>[2x]MKKNGKSQNQPLDFTQYAKNMRKDLSNQDICLEDGALNHSYFLTKKGQYWTPLNQKALQRGIELFGVGNWKEINYDEFSGKANIVELELRTCMILGINDITEYYGKKISEEEQEEIKKSNIAKGKKENKLKDNIYQKLQQMQ;>[2x]DDYLDRLPKSKKGLQGLLQDIEKRILHYKQLFFKEQNEIANGKRSMVPDNSIPICSDVTKLNFQALIDAQMRHAGKMFDVIMMDPPWQLSSSQP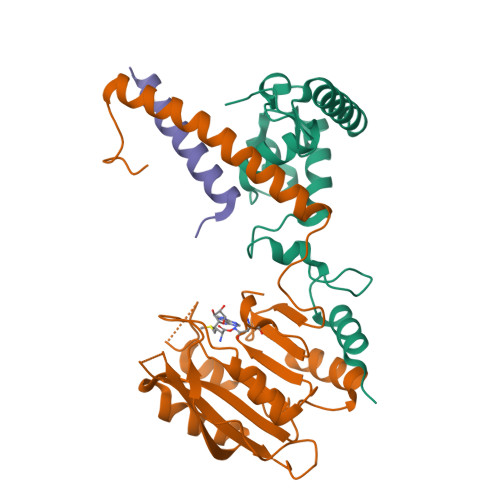SRGVAIAYDSLSDEKIQNMPIQSLQQDGFIFVWAINAKYRVTIKMIENWGYKLVDEITWVKKTVNGKIAKGHGFYLQHAKESCLIGVKGDVDNGRFKKNIASDVIFSERRGQSQKPEEIYQYINQLCPNGNYLEIFARRNNLHDNWVSIGNEL;>MSLKKGKFQHNQSKSLWNYTLSPGWREEEVKILKSALQLFGIGKWKKIMESGCLPGKSIGQIYMQTQRLLGQQSLGDFMGLQIDLEAVFNQNMKKQDVLRKNNCIINTGDNPTKEERKRRIEQNRKIYGLSAKQIAEIKLPKVKKHAPQYMTLEDIENEKFTNLEILTHLYNLKAEIVRRLAEQGETIAQPSIIKSLNNLNHNLEQNQNSNSSTETKVTLEQSGKKKYKVLAIEETELQNGPIATNSQKKSINGKRKNNRKINSDSEGNEEDISLEDIDSQESEINSEEIVEDDEEDEQIEEPSKIKKR[2x]> PKPIFREYIGVKPNSTTLHDFPTEIINTETLEFHYILGFAIESYYESGKGTGTFEESW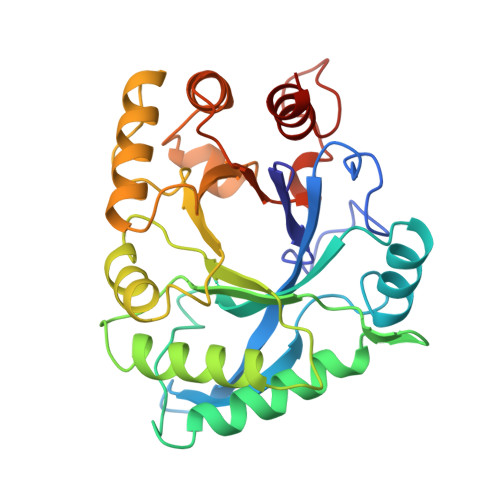DVELFGPEKVKNLKRRHPEVKVVISIGGRGVNTPFDPAEENVWVSNAKESLKLIIQKYSDDSGNLIDGIDIHYEHIRSDEPFATLMGQLITELKKDDDLNINVVSIAPSENNSSHYQKLYNAKKDYINWVDYQFSNQQKPVSTDDAFVEIFKSLEKDYHPHKVLPGFSTDPLDTKHNKITRDIFIGGCTRLVQTFSLPGVFFWNANDSVIPKRDGDKPFIVELTLQQLLAAR> RETDEEPEEPGKKGSFVEMVDNLRGKSGQGYYVEMTVGSPPQTLNILVDTGSSNFAVGAAPHPFLHRYYQRQLSST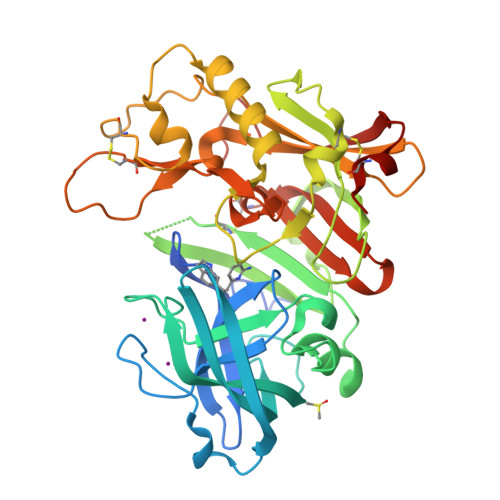YRDLRKGVYVPYTQGKWEGELGTDLVSIPHGPNVTVRANIAAITESDKFFINGSNWEGILGLAYAEIARPDDSLEPFFDSLVKQTHVPNLFSLQLCGAGFPLNQSEVLASVGGSMIIGGIDHSLYTGSLWYTPIRREWYYEVIIVRVEINGQDLKMDCKEYNYDKSIVDSGTTNLRLPKKVFEAAVKSIKAASSTEKFPDGFWLGEQLVCWQAGTTPWNIFPVISLYLMGEVTNQSFRITILPQQYLRPVEDVATSQDDCYKFAISQSSTGTVMGAVIMEGFYVVFDRARKRIGFAVSACHVHDEFRTAAVEGPFVTLDMEDCGYN> GMSREEVESLIQEVLEVYPEKARKDRNKHLAVNDPAVTQSKKCIISNKKSQPGLMTIRGCAYAGSKGVVWGPIKDMIHISHGPVGCGQYSRAGRRNYYIGTTGVNAFVTMNFTSDFQEKDIVFGGDKKLAKLIDEVETLFPLNKGISVQSECPIGLIGDDIESVSKVKGAELSKTIVPVRCEGFRGVSQSLGHHIANDAVRDWVLGKRDEDTTFASTPYDVAIIGDYNIGGDAWSSRILLEEMGLRCVAQWSGDGSISEIELTPKVKLNLVHCYRSMNYISRHMEEKYGIPWMEYNFFGPTKTIESLRAIAAKF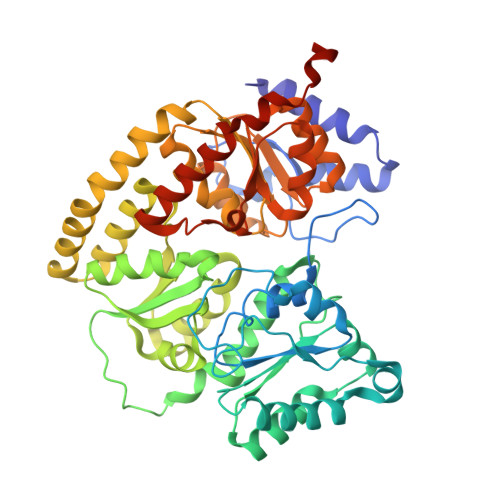DESIQKKCEEVIAKYKPEWEAVVAKYRPRLEGKRVMLYIGGLRPRHVIGAYEDLGMEVVGTGYEFAHNDDYDRTMKEMGDSTLLYDDVTGYEFEEFVKRIKPDLIGSGIKEKFIFQKMGIPFREMHSWDYSGPYHGFDGFAIFARDMDMTLNNPCWKKLQAPWEASEGAEKVAASA>GSPIGIHMSGQSLTDRITAAQHSVTGSAVSKTVCKATTHEIMGPKKKHLDYLIQCTNEMNVNIPQLADSLFERTTNSSWVVVFKSLITTHHLMVYGNERFIQYLASRNTLFNLSNFLDKSGLQGYDMSTFIRRYSRYLNEKAVSYRQVAFDFTKVKRGADGVMRTMNTEKLLKTVPIIQNQMDALLDFNVNSNELTNGVINAAFMLLFKDAIRLFAAYNEGIINLLEKYFDMKKNQCKEGLDIYKKFLTRMTRISEFLKVAE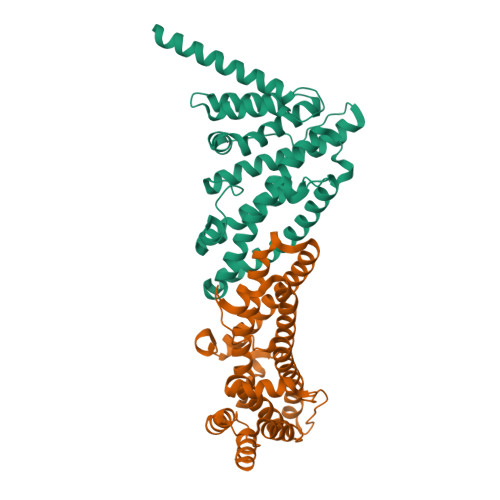QVGIDRGDI[2x]>MDHHHHHHENLYFQMEPEESMMGMKETVSNIVTSQAEKGGVKHVYYVACGGSYAAFYPAKAFLEKEAKALTVGLYNSGEFINNPPVALGENAVVVVASHKGNTPETIKAAEIARQHGAPVIGLTWIMDSPLVAHCDYVETYTFGDGKDIAGEKTMKGLLSAVELLQQTEGYAHYDDFQDGVSKINRIVWRACEQVAERAQAFAQEYKDDKVIYTVASGAGYGAAYLQSICIFMAMQWIHSACIHSGEFFHGPFEITDANTPFFFQFSEGNTRAVDERALNFLKK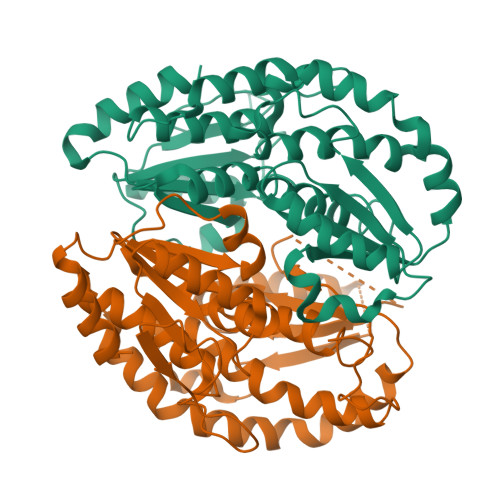YGRRIEVVDAAALGLSTIKTTVIDYFNHSLFNNVYPVYNRALAEARQHPLTTRRYMWKVEY[2x]>[2x]MAEAGITGTWYNQLGSTFIVTAGADGALTGTYESAVGNAEGDYVLTGRYDSAPATDGSGTALGWTVAWKNNYRNAHSATTWSGQYVGGAEA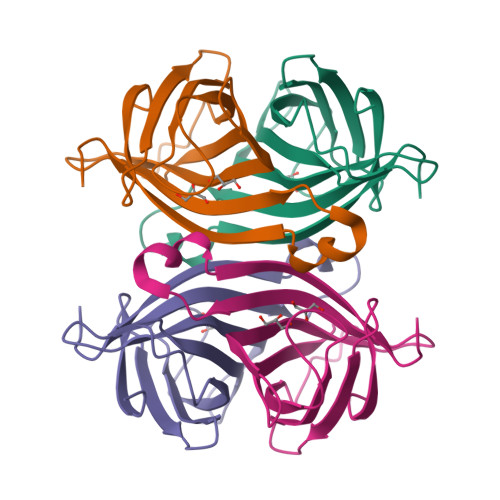RINTQWLLTSGTTEANAWKSTLVGHDTFTKVKPSAASHHHHHH> MSIKDSIGLRIKTERECQQMSREVLCLDGAELTVRQLIRIEKGESLPSLDKLSYIAKRLGKSMADLLDHDRIEIPDTYYEMKNRLIKFPTYGDKERVKQKLDLIEDVYNQFFDILPEEELLTLDILENILSFTSWEERPKVEEIYEDLFEQVKRKKKFSTNDLLVIDYYFYHLYGRKQYDKKIFDRIVDRVLKQNIPTDDAYNIALFNDLMAIAGLKISLESFKDFLTVIDKLLAVIEKSQFHSYKPGVYILEAKYELIHNGNKKKATENYDKAIMFASVLEDS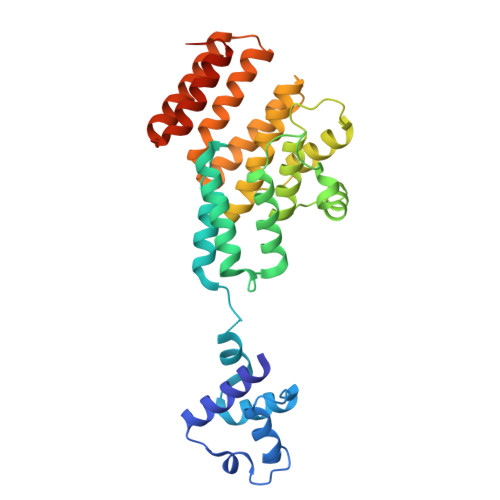VLEEKTRAEKAADGLGAGWSHPQFEK Here, we present the structural and functional elucidation of CPR-C4, a hypothetical protein from the genome of a thermophilic Candidate Phyla Radiation organism, identified through metagenomic sequencing. The function of CPR-C4 as a cysteine protease was predicted through remote structural similarity to the Homo sapiens vasohibins and subsequently confirmed experimentally with fluorescence-based activity assays. Furthermore, detailed structural and sequence alignment analysis enabled identification of a noncanonical cysteine-histidine-leucine(carbonyl) catalytic triad. In all crystal forms, the structure of CPR-C4 is a homodimer displaying a mixed αβ fold, with a central curved antiparallel β-sheet surrounded by short α-helices connected by flexible loops.

To assess the effect of the non-native His6-tag, crystallization was also subsequently conducted using protein without the tag, resulting in a third crystal form in space group P212121 and improved resolution (2.25 Å), with one dimer per asymmetric unit. Surprisingly, the two Zn2+ ions were only present in crystal form 1 and were both found to interact with the same chain (chain A), in a tetrahedral geometry, as is most common for Zn2+ coordination. However, the absence of other metal cations in the zinc-free crystal structures implies this is not a promiscuous site, and the tetrahedral ligand arrangement is strongly preferable for Zn2+ binding over other transition metal cations or the sodium and potassium present in the buffers used.

>[2x]GHMASMTGGQQMGRGSMHYKAQLQKLLTTEEKKILARLSTPQKIQDFLDTIKNKDLAEGEHTMWSPRAVLKHKHAHCMEGAMLAALALAYHGHSPLLMDLQTTDEDEDHVVALFKIDGHWGAISKTNHPVLRYRDPIYKSVRELAMSYFHEYFIWWTKKNGGKKTLRAYSNPFDLTRYKPERWVIATGDLDWLAEALDDSKHFPILNKKMQKQLRPASRIETKAASLSEWPKRKTNS> MNQDKHPEITDEEQELITVEELSQKLELLYKDMEQIRRENLLFEAYLARNRKEIAKEDEVSEDKKGKGKKKDKNVDKKSLLLTNEEKFEIAQQEQDALKKQIDDGRIKSDQILETLRAILEETDMAITEIRKDAFDFQREILVGGENSRTGKIEAEKIIKFFEEKERQKDALIAKYSSKRTNLERQILKTNNQIQKKEEMGDDLKFID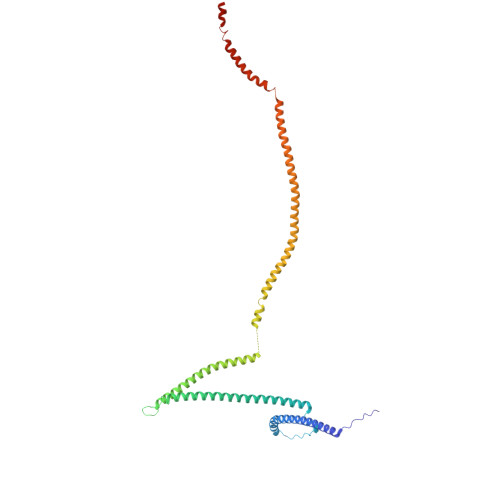FYQLQIENKKYVKEIDDKNKKLLALKISTNRISQTLKDEKQNLKQELDKGKEYASQMSERKKKISKIDAQIKSVKKVTSKLEKDRKIYDKQKEIFVQDNQDDVPQIMKYVQYKSKEQQLLYAIQNLERKIEIAELAYKKANRILQSSQQFQQK>MMYKEPFGVKVDFETGIIEGAKKSVRRLSDMEGYFVDERAWKELVEKEDPVVYEVYAVEQEEKEGDLNFATTVLYPGKVGKEFFFTKGHFHAKLDRAEVYVALKGKGGMLLQTPEGDAKWISMEPGTVVYVPVYWAHRTVNIGDEPFIFLAIYPADAGHDYGTIAEKGFSKI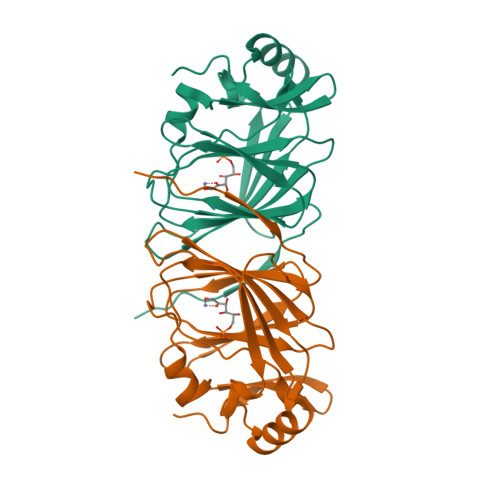VIEENGEVKVVDNPRWKK[2x]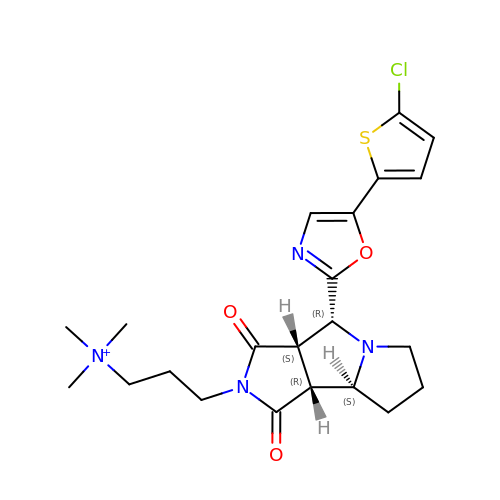3-[(3AS,4R,5S,8AS,8BR)-4-[5-(5-CHLOROTHIOPHEN-2-YL)-1,3-OXAZOL-2-YL]-1,3-DIOXO-4,6,7,8,8A,8B-HEXAHYDRO-3AH-PYRROLO[3,4-A]PYRROLIZIN-2-YL]PROPYL-TRIMETHYL-AZANIUM | C22 H28 Cl N4 O3 S | AYOZEWNCAPQIAE-ZQEOTTOMSA-N>[2x]MRDLKGIFSALLVSFNEDGTINEKGLRQIIRHNIDKMKVDGLYVGGSTGENFMLSTEEKKEIFRIAKDEAKDQIALIAQVGSVNLKEAVELGKYATELGYDCLSAVTPFYYKFSFPEIKHYYDTIIAETGSNMIVYSIPFLTGVNMGIEQFGELYKNPKVLGVKFTAGDFYLLE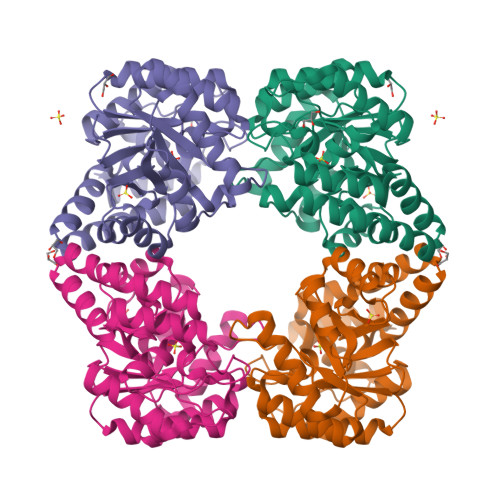RLKKAYPNHLIWAGFDEMMLPAASLGVDGAIGSTFNVNGVRARQIFELTKAGKLKEALEIQHVTNDLIEGILANGLYLTIKELLKLEGVDAGYCREPMTSKATAEQVAKAKDLKAKFLS> ASTPVFWDDPQNHTFRHTLFCQDGIPNIGLSETYDEDELFSFDFSQNTRVPRLPDFAEWAQGQGDASAIAFDKSFCEMLMREVSPKLEGQIPVSRGLPVAEVFTLKPLEFGKPNTLVCFISNLFPPTLTVNWQLHSAPVEGASPTSISAVDGLTFQAFSYLNFTPEPFDLYSCTVTHEI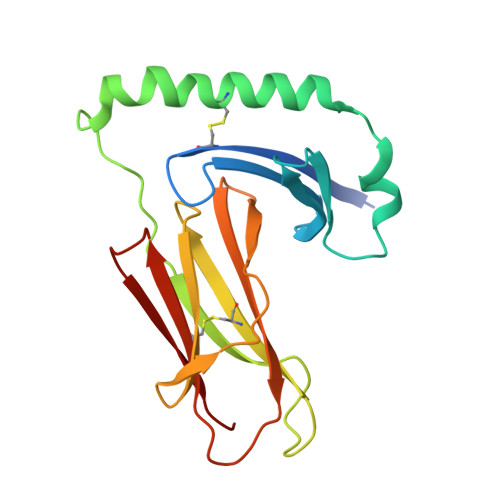DRYTAIAYWVPQ> HSPEEQKQMLGEAIYPKVAASQPELAGKLTGMILELPVTELLHLLEESEALDAKVNE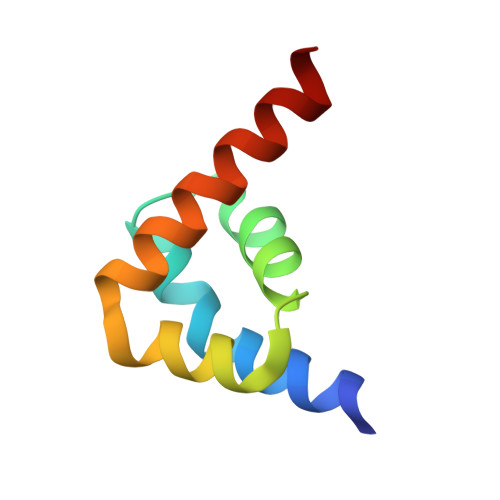ALEVLKEYQQN>ASEIELVFRPHPTLMEKDDSAQTRYIKTSGNATVDHLSKYLAVRLALEELRSKGESNQMNLDTASEKQYTIYIATASGQFTVLDGSFSLELVSEKYWKVNKPMELYYAPTK[6x];>GTRPRLKNVDRSTAQQLAVT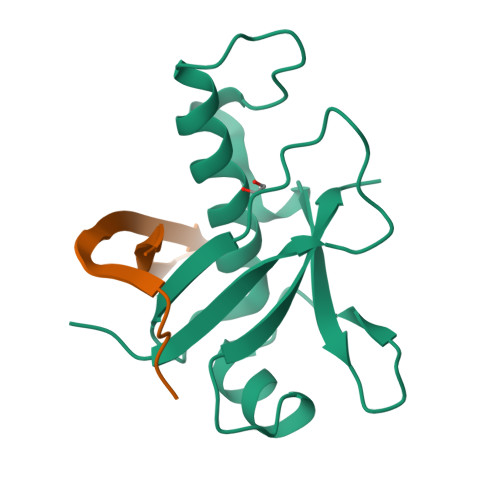VGNVTVIITDFKEKTRS[6x]>[2x]MAPLQPGDSFPANVVFSYIPPTGSLDLTVSGRPIEYNASEALAKGTSVLVAVPGAFTPTCQEKHVTGFIAKLDQLRQAGVDRVLFIASNDAFVMSA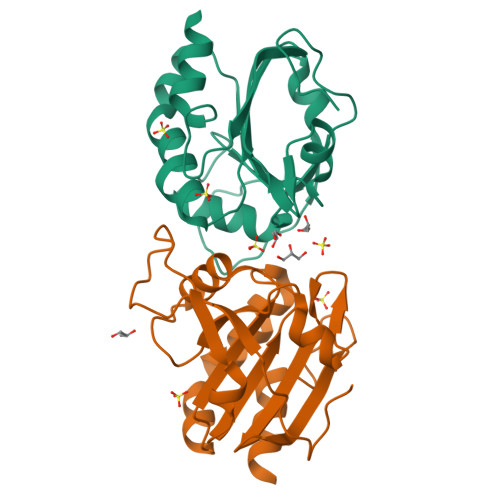WGKANGIKDESILFLSDSDTAFSSSIGWANAGRTGRYAIVVKDGKVVYAAVDTVRGSTEKSGVDAVLTVLGNQGKL>[8x]MASQVGAINSVNALISRVFVQPKGDLADRLNSRVTVVILAVSSALLLSSHFIGDPITCWTPAQFNAQWVNFVNQYCFVHGTYFVPLDQQLAFEEEERTKVSIQYYQWVPYVFALQAFLFYIPRFIWKAMIAYSGYDLAAAVKYVDRFWSENRDKDDKFKTRLAAFEGRPSVYIWDGIRLARKKRSRNMALFYTLSTVWQAVNAWIQFYILTQLLDSSIYTLWGPSILGDLLQGNDWQTTGHFPRIVHCDFNRRRPASVQLDTVLCVLTLNIYYEKLFIFLWFWLVFVAVVSTVNCFKWIYYLCNKTKAQKTIKNYLSTAPIKSTISDDQFFSALGEDGLFIMDQMALNLGDIPASYLTISMRNICQDFIESEDYIDEERTPFVKSIKHT

Invertebrates possess a different gap junction protein family, termed innexins, that is essential for eating and developmental functions in Caenorhabditis elegans and for electrical synapses in Drosophila7. We recently revealed that the C. elegans innexin-6 (INX-6) gap junction channel structure is a 16-subunit oligomer, that is, a hexadecamer, with larger dimensions than those of connexins. Here we report the atomic resolution structures of INX-6 determined by cryo-EM in combination with GraDeR.

We first attempted to reconstruct a hemichannel of INX-6 as semi-auto particle picking worked very well. A three-dimensional map was reconstructed from 74,398 particles with C8 symmetry, and the final resolution after refinement was 3.3 Å, which was sufficient for de novo model building. The map of the INX-6 hemichannel includes part of the densities of the extracellular domains of an opposed hemichannel. The Met1 to Gly6 residues at the N-terminal end, Ile52 and Gly53 following TM1, and Glu370 to the C-terminal end were not assigned due to the disorder of the structure. Two helices (CLH1 and CLH2) in CL and four helices (CTH1 to CTH4) in CT are arranged in a helix-turn-helix motif, aligning vertically to form a cytoplasmic core. The INX-6 structure is divided into three parts: the cytoplasmic dome, the transmembrane region including a pore funnel and the extracellular gap region. In the cytoplasmic dome, the CLs and CTs are intercalated one by one through the eight subunits, creating a dome-shaped pore entrance with a 30-Å diameter (Fig. 4b—cytoplasmic). The inter-subunit interfaces are reinforced by the polar interactions of Arg168-Asp153, Asp175-Tyr356, Arg178-Thr318, Lys182-Ser317 and Lys183-Asp351, resulting in a roof made of consecutively placed cytoplasmic cores. We found additional densities inserted into the inter-subunit space. These densities could be assigned to lipids carried over during purification, which may serve to stabilize the transmembrane bundles and may also contribute to the conformation of the N-terminal funnel due to the proximity. The N-terminal loops are harnessed by the cytoplasmic dome, and the disordered Ile52 and Gly53 cause the flexibility of TM1 in the pore cavity.> MDQGEFIQDDNDQDYDQQEGDDENNDYMEDPQQDNNYNQNGDNLDDQGQDDDGGQNNLQQPSVPPEDDEDDDDDFPEYANEQNKRLNEIIKKKRKLIKDISAKIEEKSDRTKVLQEHLKNVEQELLHTQALIDAKNKEIETEDHMKQIAERQSGRIQSELKILEKRSIEQQEKLNDVQNQIFRGNEKMDQYKLEMNWNQEELEQWALAARQKEEDNLTLEKYKRADEVKIKELNLAIEKLTAEVGRKQNELEKEITETQAAQIELDKTAEEFKRQHEERHKLFLQWQEVTEIISKRDLAIREEGENFARIKIEIKSNKDALEERKRILKEAKEENKRIQMANELMERQNIQQISDNKHIEEQLAEKKADVEILKNQVSAFASDLSSKKNRIAILSQELLAKKQRLNAAQKKYQAHQVKLKNEEIMAKQYENDRSYAEEKYRKNEKEKKELEKEIRTQKENLFKHTQELFKHRERE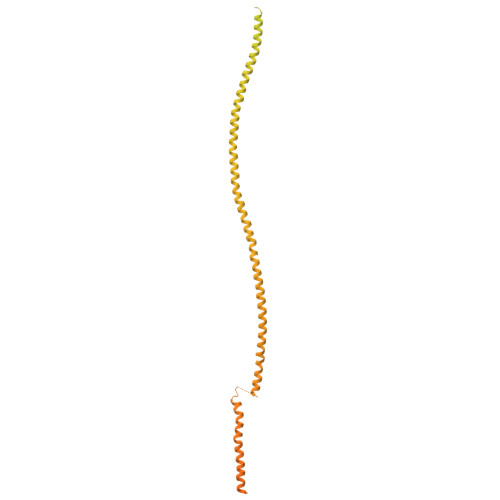ANLYGEIQGNMAACRNLQSHITKLNQEFQRQQELLYNAEYQIQLMERRVARAKGERTLEEKKDLENEIMNAERELGGVTGQNKELIESLKNLDDEIRTVKKKLAYVEEENTKYSSLIEELILENDMTYQDLNKIIKQKEEVLVQHDTMKLEIKKINESLNGATEKVFNLENQIYQLEMSMQEREKEIEVHKDVLMTEHKAAEEERHKIAVELAERKNKVKNLKIKYESLVQKNKASNGEVESVHEHSQAYYVIKAAQEREELQRKGDELNAKILKNEKELKALDNTLNHLKNRNSNYRDKFLNKGVTTQHREEAEGLEEQCRAASQNLFKKRDELQKLQKEQEEDTRRYTEIKNKLERLYEQHQSLDQEISKYQKDIDQQGDKLQRAQNSLQRNYQLAVNKNQNFINPKNPHMIQVKLDNQNNLYKTLLQGLYSLQQDIPELSSVVDEILKEQRIQNNKAPSSIDINSKRSSQSGRSQRSQRSNISNQ>RKPKTGILMLNMGGPETLGDVHDFLLRLFLDRDLMTLPIQNKLAPFIAKRLTPKIQEQYRRIGGGSPIKIWTSKQGEGMVKLLDELSPNTAPHKYYIGFRYVHPLTEEAIEEMERDGLERAIAFTQYPQYSCSTTGSSLNAIYRYYNQVGRKPTMKWSTIDRWPTHHLLIQCFADHILKELDHFPLEKRSEVVILFSACSLPMSVVNRGDPYPQEVSATVQKVMERLEYCNPYRLVWQSKVGPMPWLGPQTDESIKGLCERGRKNILLVPIAFTSDHIETLYELDIEYSQVLAKECGVENIRRAESLNGNPLFSKALADLVHSHIQSNELCSKQLTLSCPL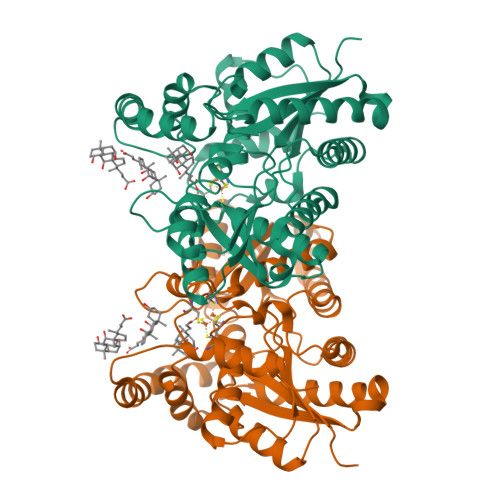CVNPVCRETKSFFTSQQL[2x]>[2x]MAHHHHHHMSQEITLGNIKIGGNNPVFIIAEAGLNHGGDLNLALRMIDEAADAKANAIKFQAYNSEERFGENKEAVNLVKPAE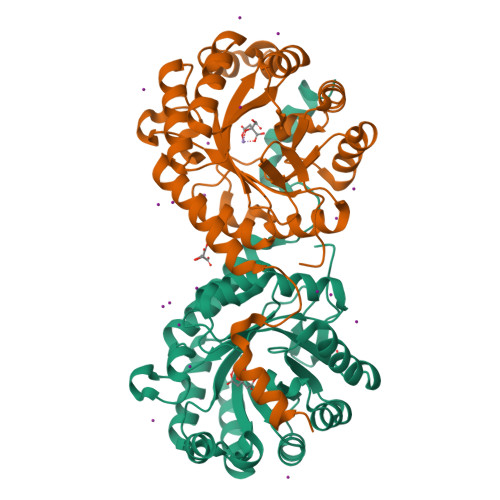FGKKEFLLLKERSQKKNILFFATPFDVPNLNMLKEIGVEILKIASCDICNITLLEAAADSGLIVILSRGTASASEIETAVSIFKKKKSPFILLHCVSSYPMNEIDANLSAIQTLKSKYEFPIGYSDHSKGIEIPLLAVASGAEIIEKHYTVDRTLQGIDWEISAEPKELAKLVTETERIRKILGHGKLEPQASEQEEIEYRNSLRRK> YTPVAVQCQEAQLVVTVHRDLFGTGRLINAADLTLGPAACKHSSLNAAHNTVTFAAGLHECGSVVQVTPDTLIYRTLINYDPSPASNPVIIRTNPAVIPIECHYPRREQVSSNAIRPTWSPFNSALSAEERLVFSLRLMSDDWSTERPFTGFQLGDILNIQAEVSTENHVPLRLFVDSCVAALSPDGDS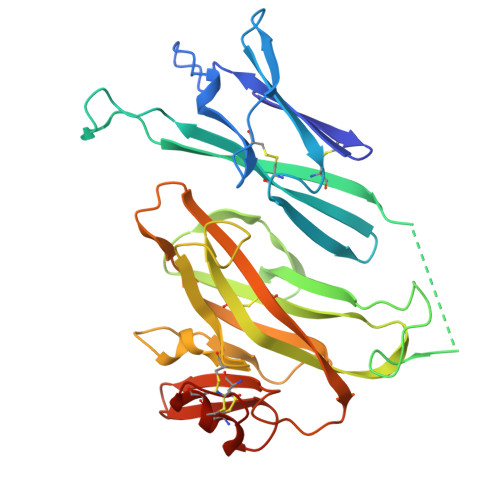SPHYAIIDFNGCLVDGRVDDTSSAFITPRPREDVLRFRIDVFRFAGDNRNLIYITCHLKVTPADQGPDPQNKACSFNKARNTWVPVEGSRDVCNCCETGNCEPPALSR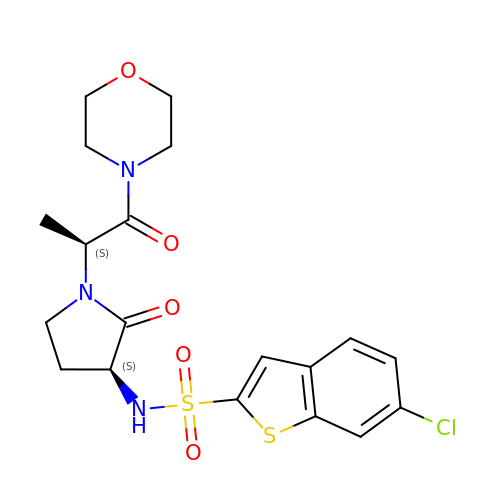6-CHLORO-N-{(3S)-1-[(1S)-1-METHYL-2-MORPHOLIN-4-YL-2-OXOETHYL]-2-OXOPYRROLIDIN-3-YL}-1-BENZOTHIOPHENE-2-SULFONAMIDE | C19 H22 Cl N3 O5 S2 | PHLKBODTBJLXRD-WFASDCNBSA-N> MDDLTLRYFDAEMRYLREAGKAFAQAHPDRAAMLDLDKAGTPDPCVERLFEGFAFSMGRLRQKIDDDLPELTESLVSMLWPHYLRTIPSLSVVALTPRLSVMKMAETVPAGLEVTSRPVGPGNTVCRYRTTRAIPLNPLAVEKVVMTTEPDGRSVLKIGFACSELADWSQVDLHRLSLYLAAEAPVSSTLHLMMTKRLAALYLRLPGNDERIRIDGWFSPGGFAEEDRLWPKGDSAFSGYQLLLEYFTFREKFMFVHLNGLENVSLPAGISGFDLEVVLSQPWPADLPVTDDALCLHCVPVINLFTLEADPLIINGLESEYLLRPKRLQDGYTEIYSVDAVTGSGRTGSAEYVPFTSFRHRGGMLRHDAPERYYHTRVKR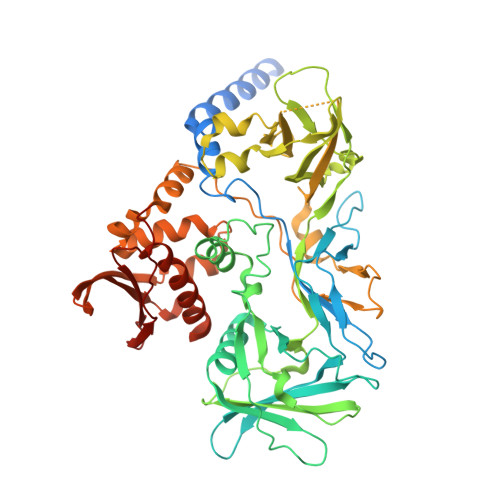GVTGMYDTWLILGGQRWEADRMPERETLSLRITGTNGQLPRRALQSTLLDRCEQVLQAPVSVRNLCKPTLPVYPPTEDRFHWRVMSHLGTGFLNMLSSAEVLRGTLALYNWRDDELNHRRLDAILAVQHHRIQRFEKGFLLRGLDVEVTLDGNGFAGEGDIHLFGEMLNRFLALYADMNQFNQLTLIVQPEGKCIRWKENHNPRLPG> SMSLVPATNYIYTPLNQLKGGTIVNVYGVVKFFKPPYLSKGTDYCSVVTIVDQTNVKLTCLLFSGNYEALPIIYKNGDIVRFHRLKIQVYKKETQGIT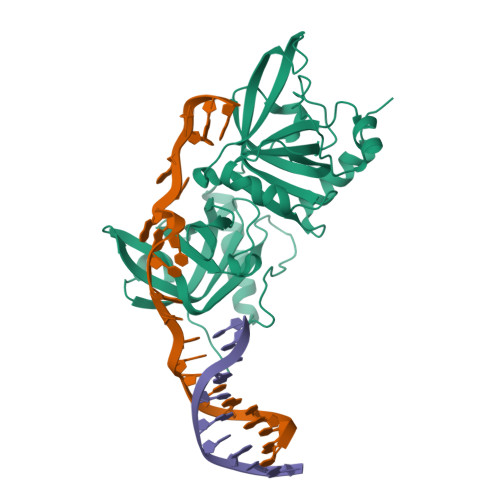SSGFASLTFEGTLGAPIIPRTSSKYFNFTTEDHKMVEALRVWASTHMSPSWTLLKLCDVQPMQYFDLTCQLLGKAEVDGASFLLKVWDGTRTPFPSWRVLIQDLVLEGDLSHIHRLQNLTIDILVYDNHVHVARSLKVGSFLRIYSLHTKLQSMNSENQTMLSLEFHLHGGTSYGRGIRVLPESNSDVDQLKKDLESANLTA>[2x]QSLRSSLLGLRQLLRELPGDEAPLDALAETVLALLAQYGSLRIAGLYRVRYDRTPEPQPLATLGEMPALDADDLLVRTCLERGELVSVRQELLERGEQRAHSALQVCVPLVDTDGRILALLAVEQMPFFVFNERTFSLLAILAGHIADLLQSDRRALQLADIDAQRFSQYLKRSLLDARDHGLPAC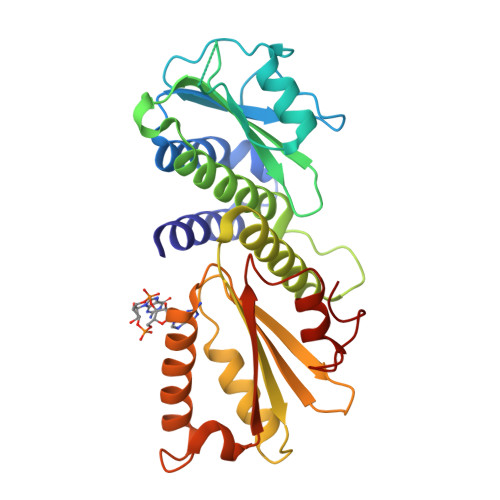LYAFELTDARYGEEVQRLLEGSQRGLDVQLRLRNDEGRRVLLVLLPLTSAEGSQGYLQRLRILFAERFGQARELESLGVRIRQYELDAGNDRQALGHFLFNECGLNDQQVA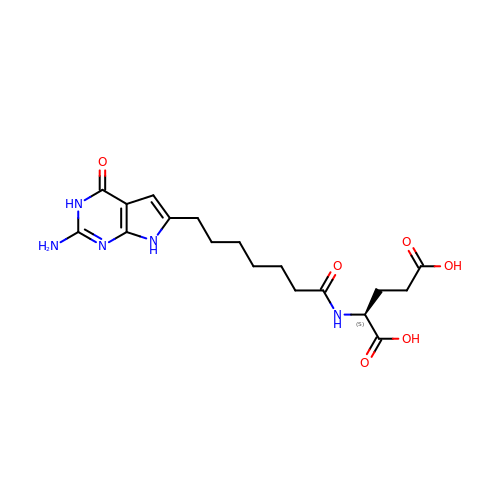(S)-2-(7-(2-Amino-4-oxo-4,7-dihydro-3H-pyrrolo[2,3-d]pyrimidin-6-yl)heptanamido)pentanedioic acid | C18 H25 N5 O6 | YFTJOYZLYVUUOD-LBPRGKRZSA-N> DEDGLISLIFNKKESDIRGQQQ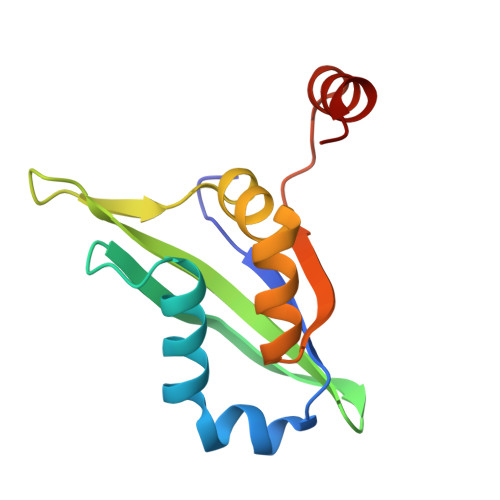QLVESLHKVLGGHQTLTVNVEGVKTKADNQTEVIIYVVERSPNGTSRRVGASALFSYFEQAHIKANMQSLGVTGAMAQTELSPVQIKQLIQNPL>MLASLEARYPGLAFAWPRPGVLEITFRGEKLNAMPPALHRGLARVWRDLEAVEGVRAVLLRGEGGVFSAGGSFGLIEEMRA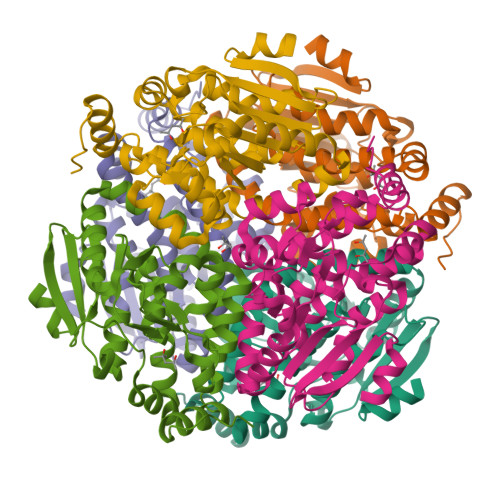SHEALLRVFWEARDLVLGPLNFPRPVVAAVEKVAVGAGLALALAADIAVVGKGTRLLDGHLRLGVAAGDHAVLLWPLLVGMAKAKYHLLLNEPLTGEEAERLGLVALAVEDEKVYEKALEVAERLAQGPKEALHHTKHALNHWYRSFLPHFELSLALEFLGFSGKELEEGLKALKEKRPPEFP[6x]> XPIPFLS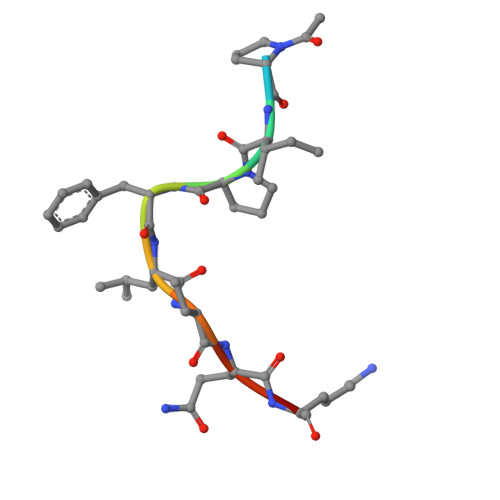QKD>MRRETVGEFSSDDDDDILLELGTRPPRFTQIPPSSAALQTQIPTTLEVTTTTLNNKQSKNDNQLVNQLNKAQGEASMLRDKINFLNIEREKEKNIQAVKVNELQVKHLQELAKLKQELQKLEDEKKFLQMEARGKSKREVITNVKPPSTTLSTNTNTITPDSSSVAIEAKPQSPQSKKRKISDNLLKKNMVPLNPNRIIPDETSLFLESILLHQIIGADLSTIEILNRLKLDYITEFKFKNFVIAKGAPIGKSIVSLLLRCKKTLTLDRFIDTLLEDIAVLIKEISVHPNESKLAVPFLVALMYQIVQFRPSATHNLALKD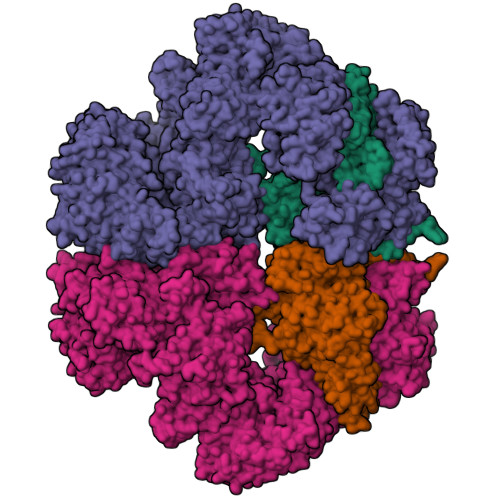CFLFICDLIRIYHHVLKVPIHESNMNLHVEPQIFQYELIDYLIISYSFDLLEGILRVLQSHPKQTYMEFFDENILKSFEFVYKLALTISYKPMVNVIFSAVEVVNIITSIILNMDNSSDLKSLISGSWWRDCITRLYALLEKEIKSGDVYNENVDTTTLHMSKYHDFFGLIRNIGDNELGGLISKLIYTDRLQSVPRVISKEDIGMDSDKFTAPIIGYKMEKWLLKLKDEVLNIFENLLMIYGDDATIVNGEMLIHSSKFLSREQALMIERYVGQDSPNLDLRCHLIEHTLTIIYRLWKDHFKQLREEQIKQVESQLIMSLWRFLVCQTETVTANEREMRDHRHLVDSLHDLTIKDQASYYEDAFEDLPEYIEEELKMQLNKRTGRIMQVKYDEKFQEMARTILESKSFDLTTLEEADSLYISMGL[2x];>[2x]MESHVKYLDELILAIKDLNSGVDSKVQIKKVPTDPSSSQEYAKSLKILNTLIRNLKDQRRNNIMKNDTIFSKTVSALALLLEYNPFLLVMKDSNGNFEIQRLIDDFLNISVLNYDNYHRIWFMRRKLGSWCKACVEFYGKPAKFQLTAHFENTMNLYEQALTEVLLGKTELLKFYDTLKGLYILLYWFTSEYSTFGNSIAFLDSSLGFTKFDFNFQRLIRIVLYVFDSCELAALEYAEIQLKYISLVVDYVCNRTISTALDAPALVCCEQLKFVLTTMHHFLDNKYGLLDNDPTMAKGILRLYSLCISNDFSKCFVDHFPIDQWADFSQSEHFPFTQLTNKALSIVYFDLKRRSLPVEALKYDNKFNIWVYQSEPDSSLKNVTSPFDDRYKQLEKLRLLVLKKFNKTERGTLLKYRVNQLSPGFFQRAGNDFKLILNEASVSIQTCFKTNNITRLTSWTVILGRLACLESEKFSGTLPNSTKDMDNWYVCHLCDIEKTGNPFVRINPNRPEAAGKSEIFRILHSNFLSHPNIDEFSESLLSGILFSLHRIFSHFQPPKLTDGNGQINKSFKLVQKCFMNSNRYLRLLSTRIIPLFNISDSHNSEDEHTATLIKFLQSQKLPVVKENLVIAWTQLTLTTSNDVFDTLLLKLIDIFNSDDYSLRIMMTLQIKNMAKILKKTPYQLLSPILPVLLRQLGKNLVERKVGFQNLIELLGYSSKTILDIFQRYIIPYAIIQYKSDVLSEIAKIMCDGDTSLINQMKVNLLKKNSRQIFAVALVKHGLFSLDILETLFLNRAPTFDKGYITAYLPDYKTLAEITKLYKNSVTKDASDSENANMILCSLRFLITNFEKDKRHGSKYKNINNWTDDQEQAFQKKLQDNILGIFQVFSSDIHDVEGRTTYYEKLRVINGISFLIIYAPKKSIISALAQISICLQTGLGLKEVRYEAFRCWHLLVRHLNDEELSTVIDSLIAFILQKWSEFNGKLRNIVYSILDTLIKEKSDLILKLKPYTTLALVGKPELGILARDGQFARMVNKIRSTTDLIPIFANNLKSSNKYVINQNLDDIEVYLRRKQTERSIDFTPKKVGQTSDITLVLGALLDTSHKFRNLDKDLCEKCAKCISMIGVLDVTKHEFKRTTYSENEVYDLNDSVQTIKFLIWVINDILVPAFWQSENPSKQLFVALVIQESLKYCGLSSESWDMNHKELYPNEAKLWEKFNSVSKTTIYPLLSSLYLAQSWKEYVPLKYPSNNFKEGYKIWVKRFTLDLLKTGTTENHPLHVFSSLIREDDGSLSNFLLPYISLDIIIKAEKGTPYADILNGIIIEFDSIFTCNLEGMNNLQVDSLRMCYESIFRVFEYCKKWATEFKQNYSKLHGTFIIKDTKTTNMLLRIDEFLRTTPSDLLAQRSLETDSFERSALYLEQCYRQNPHDKNQNGQLLKNLQITYEEIGDIDSLDGVLRTFATGNLVSKIEELQYSENWKLAQDCFNVLGKFSDDPKTTTRMLKSMYDHQLYSQIISNSSFHSSDGKISLSPDVKEWYSIGLEAANLEGNVQTLKNWVEQIESLRNIDDREVLLQYNIAKALIAISNEDPLRTQKYIHNSFRLIGTNFITSSKETTLLKKQNLLMKLHSLYDLSFLSSAKDKFEYKSNTTILDYRMERIGADFVPNHYILSMRKSFDQLKMNEQADADLGKTFFTLAQLARNNARLDIASESLMHCLERRLPQAELEFAEILWKQGENDRALKIVQEIHEKYQENSSVNARDRAAVLLKFTEWLDLSNNSASEQIIKQYQDIFQIDSKWDKPYYSIGLYYSRLLERKKAEGYITNGRFEYRAISYFLLAFEKNTAKVRENLPKVITFWLDIAAASISEAPGNRKEMLSKATEDICSHVEEALQHCPTYIWYFVLTQLLSRLLHSHQSSAQIIMHILLSLAVEYPSHILWYITALVNSNSSKRVLRGKHILEKYRQHSQNPHDLVSSALDLTKALTRVCLQDVKSITSRSGKSLEKDFKFDMNVAPSAMVVPVRKNLDIISPLESNSMRGYQPFRPVVSIIRFGSSYKVFSSLKKPKQLNIIGSDGNIYGIMCKKEDVRQDNQYMQFATTMDFLLSKDIASRKRSLGINIYSVLSLREDCGILEMVPNVVTLRSILSTKYESLKIKYSLKSLHDRWQHTAVDGKLEFYMEQVDKFPPILYQWFLENFPDPINWFNARNTYARSYAVMAMVGHILGLGDRHCENILLDIQTGKVLHVDLDCLFEKGKRLPVPEIVPFRLTPNLLDALGIIGTEGTFKKSSEVTLALMRKNEVALMNVIETIMYDRNMDHSIQKALKVLRNKIRGIDPQDGLVLSVAGQTETLIQEATSEDNLSKMYIGWLPFW>GAPIHDPDFIGGIGKELIVDNASDVTSFYPSAFQEHLNFIPAPTTGSGCTRIPSFDMSATHYCYTHNVILSGCRDHSHSHQYLALGVLRTTATGRIFFSTLRSISLDDTQNRKSCSVSATPLGCDMLCSKVTETEEEDYNSAVPTLMAHGRLGFDGQYHEKDLDVTTLFEDWVANYPGVGGGSFIDGRVWFSVYGGLKPNSPSDTVQEGKYVIYKRYNDTCPDEQDYQIRMAKSSYKPGRFGGKRIQQAILSIKVSTSLGEDPVLTVPPNTVTLMGAEGRILTVGTSHFLYQRGSSYFSPALLYPMTVSNKTATLHSPYTFNAFTRPGSIPCQASARCPNSCVTGVYTDPYPLIFYRNHTLRGVFGTMLDSEQARLNPASAVFDSTSRSRITRVSSSSTKAAYTTSTCFKV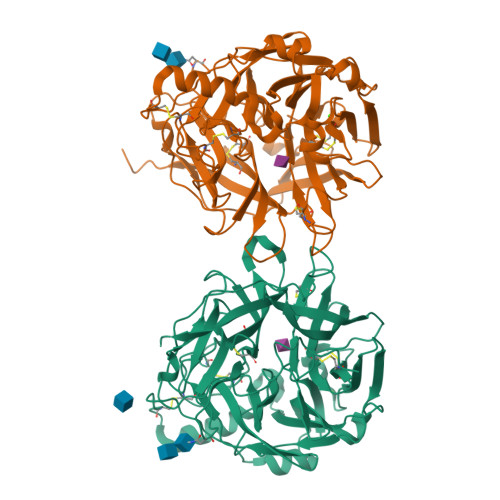VKTNKTYCLSIAEISNTLFGEFRIVPLLVEILKNDGVREARSG[2x]> CPQEDSDIAFLIDGSGSIIPHDFRRMKEFVSTVMEQLKKSKTLFSLMQYSEEFRIHFTFKEFQNNPNPRSLVKPITQLLGRTHTATGIRKVVRELFNITNGARKNAFKILVVITDGEKFGDP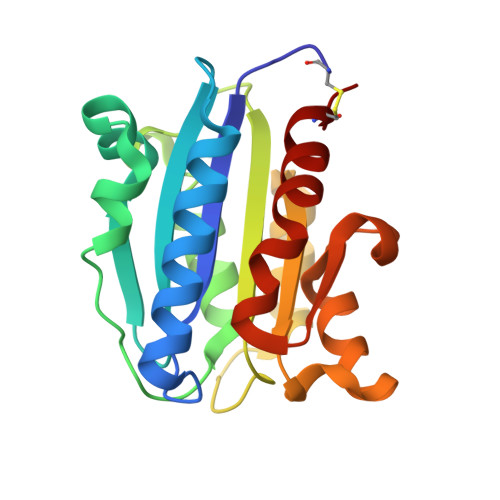LGYEDVIPEADREGVIRYVIGVGDAFRSEKSRQELNTIASKPPRDHVFQVNNFEALKTIQNQLREKIFCIGS> DKMDYDFKVKLSSERERVEDLFEYEGCKVGRGTYGHVYKAKRKDGKDDKDYALKQIEGTGISMSACREIALLRELKHPNVISLQKVFLSHADRKVWLLFDYAEHDLWHIIKFHRASKANKKPVQLPRGMVKSLLYQILDGIHYLHANWVLHRDLKPANILVMGEGPERGRVKIADMGFARLFNSPLKPLADLDPVVVTFWYRAPELLLGARHYTKAIDIWAIGCIFAELLTSEPIFHCRQEDIKTSNPYHHDQLDRIFNVMGFPADKDWEDIKKMPEHSTLMKDFRRNTYTNCSLIKYMEKHKVK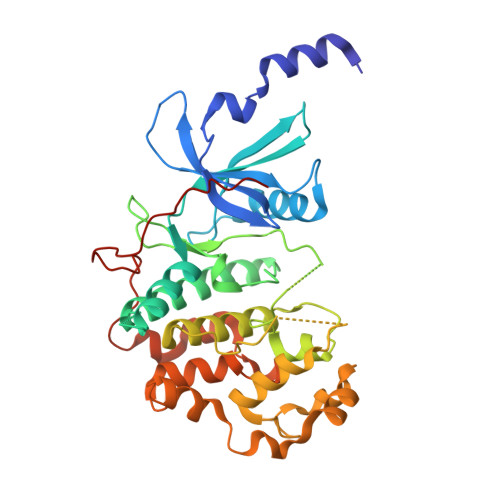PDSKAFHLLQKLLTMDPIKRITSEQAMQDPYFLEDPLPTSDVFAGCQIPYPKREFLTEEEPPLKK>MESYNIAVLAGDGIGPEVMAEAIKVLNRVQEKFGFKLNFNEFFVGGAAIEHCGYPLPAETLKGCDQADAILFGSVGGPKWTNLPPDQQPERGALLPLRKHFKLFCNLRPATLYKGLEKFCPLRADIAAKGFDMVVVRELTGGIYFGQPKGREGDGVQTKAFDTEVYYKYEIERIARAAFEAAMKRNKKVTSVDKANVLQSSILWRETVTEMAKDYPEVTLEHIYIDNATMQLIKSPESFDVLLCSNIFGDIISDEAAMITGSMG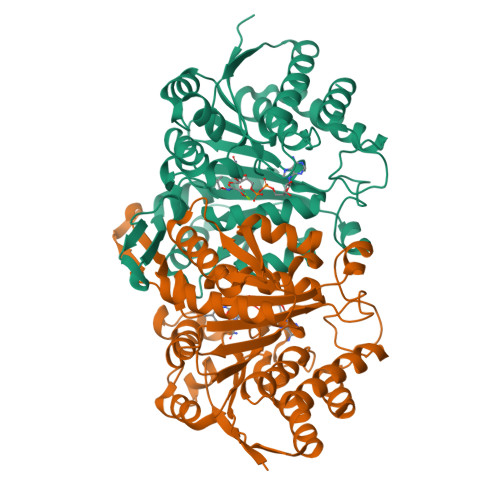MLPSASLNEEGFGLYEPAGGSAPDIAGKGIANPIAQILSAAMMLRYSFNLNEAADAIESAVQKVLASGHRTADLADDSTPVSTAEMGTLITQAI[2x]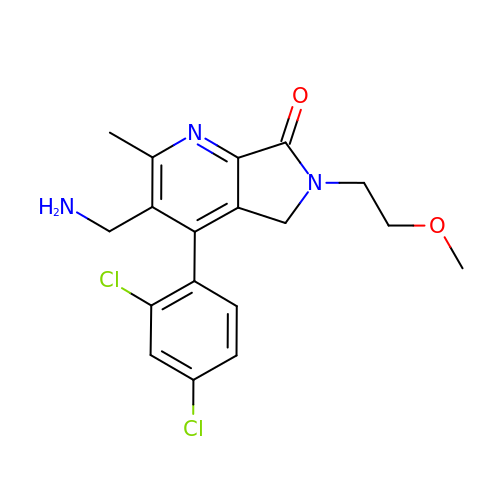3-(aminomethyl)-4-(2,4-dichlorophenyl)-6-(2-methoxyethyl)-2-methyl-5,6-dihydro-7H-pyrrolo[3,4-b]pyridin-7-one | C18 H19 Cl2 N3 O2 | CLNAIMPDNPYUGV-UHFFFAOYSA-N> MQTGFNLSIDTVEGNPGSSVV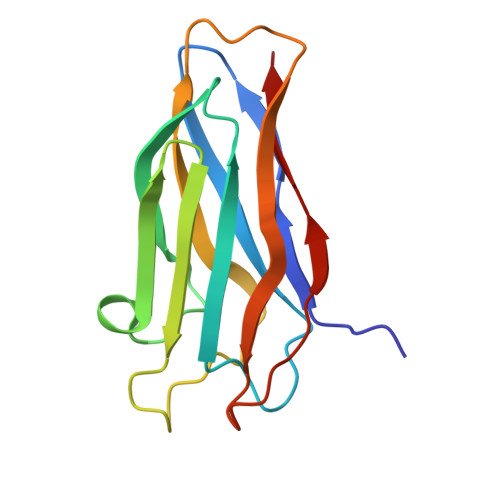VPVKLSGISKNGISTADFTVTYDATKLEYISGDAGSIVTNPGVNFGINKESDGKLKVLFLDYTMSTGYISTDGVFANLNFNIKSSAAIGSKAEVSISGTPTFGDSTLTPVVAKVTNGAVNLE S-[2-(acetylamino)ethyl] 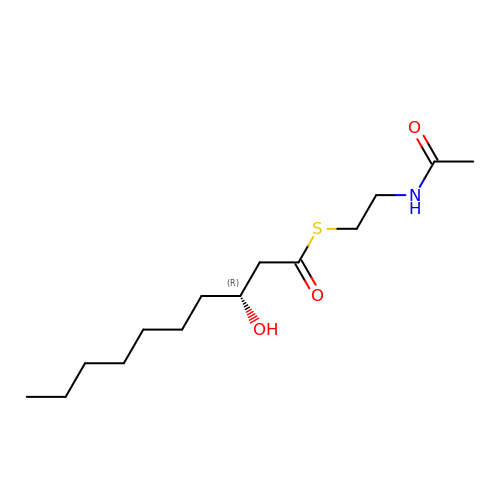(3R)-3-hydroxydecanethioate | C14 H27 N O3 S | AKKZYNFGIOAWKB-CYBMUJFWSA-N> MAKHPTPMLDELEKGPWPSFVSDIKQECDNRAKNPKGLDYQIPAECPDDLLGILELSFHEGETHWKHGGIVGVFGYGGGVIGRYCDQPEMFPGVAHFHTVRLAQPAAKYYTAEYLEAICDVWDLRGSGLTNMHGSTGDIVLLGTQTPQLEEIFFEMTHNLNTDLGGSGSNLRTPESCLGISRCEFACYDTQLMCYQLTQDYQDELHRPAFPYKFKF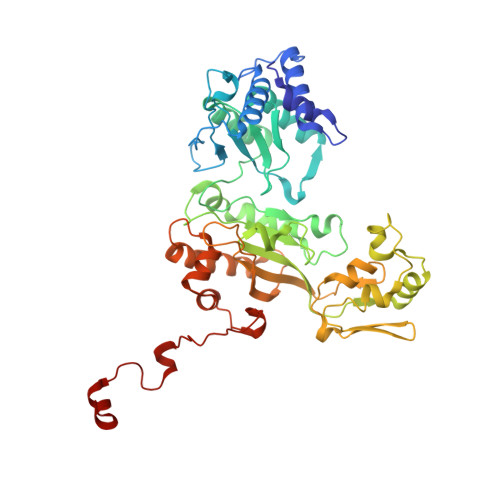KFDGCPNGCVASMARSDFAVIGTWKDDIKIDQEAVKAYVGGEFKPNAGAHAGRDWGKFDIEAEVVGLCPTGCMTYESGTLSIDNKNCTRCMHCINTMPRALKIGDERGASILVGAKAPVLDGAQMGSLLIPFIAAEEPFDEVKEVIENIWEWWMEEGKNRERLGETMKRVGFQKLLEVTGTKAVPQHVSEPRHNPYIFFKEEEVPGGWSRDISDYRKRHMR>MGSRASTLLRDEELEEIKKETGFSHSQITRLYSRFTSLDKGENGTLSREDFQRIPELAINPLGDRIINAFFSEGEDQVNFRGFMRTLAHFRPIEDNEKSKDVNGPEPLNSRSNKLHFAFRLYDLDKDDKISRDELLQVLRMMVGVNISDEQLGSIADRTIQEADQDGDSAISFTEFVK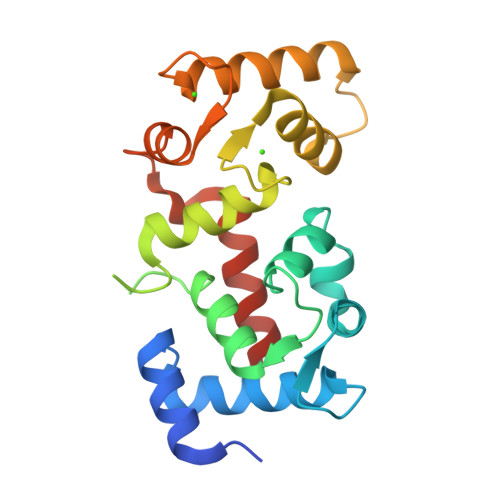VLEKVDVEQKMSIRFLHKLAAALEHHHHHH[2x]>[6x]CDLPQTHSLGSRRTLMLLAQMRRISLFSCLKDRHDFGFPQEEFGNQFQKAETIPVLHEMIQQIFNLFSTKDSSAAWDETLLDKFYTELYQQLNDLEACVIQGVGVTETPLMNEDSILAVR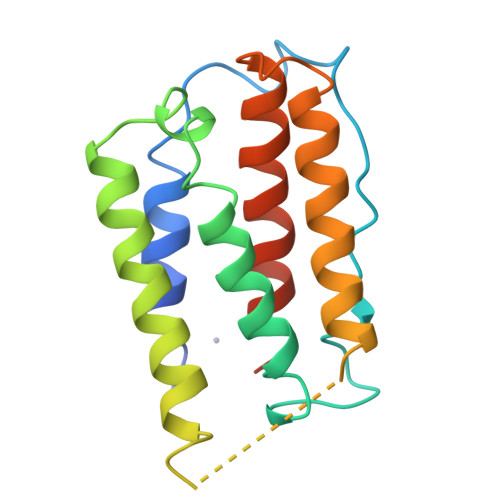KYFQRITLYLKEKKYSPCAWEVVRAEIMRSFSLSTNLQESLRSKE>GPHMTDKSDRTDWVALMRAIRDHRDEAAFAELFQHFAPKVKGFLMKSGSVASQAEECAQDVMATVWQKAHLFDPSRASVATWIFTIARNRRIDGLRKDRQPEPEDLFWGPDSEPDQADVYEMQQENARLGRAIARLPEAQRALIERAFFGDLTHRELAAETGLPLGTIKSRIRLALDRLRQHMS[4x];>MTIRHHVSDALLTAYAAGTLSEAFSLVVATHLSLCDECRARAGALDAVGGSLMEETAPVALSEGSLASVMAQLDRQIQRPAPARRADPRAPAPLADYVGRRLEDVRWRTLGGGV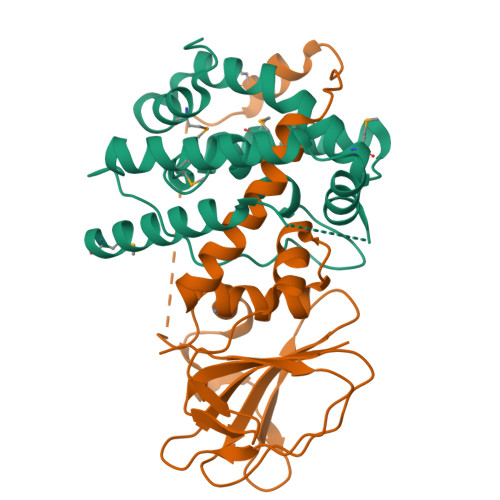RQAILPTGGEAIARLLWIPGGQAVPDHGHRGLELTLVLQGAFRDETDRFGAGDIEIADQELEHTPVAERGLDCICLAATDAPLRFNSFL[4x]>MEAVPRMPMIWLDLKEAGDFHFQPAVKKFVLKNYGENPEAYNEELKKLELLRQNAVRVPRDFEGCSVLRKYLGQLHYLQSRVPMGSGQEAAVPVTWTEIFSGKSVAHEDIKYEQACILYNLGALHSMLGAMDKRVSEEGMKVSCTHFQCAAGAFAYLREHFPQAYSVDMSRQILTLNVNLMLGQAQECLLEKSMLDNRKSFLVARISAQVVDYYKEACRALENPDTASLLGRIQKDWKKLVQMKIYYFAAVAHLHMGKQAEEQQKFGERVAYFQSALDKLNEAIKLAKGQPDTVQDALRFTMDVIGGKYNSA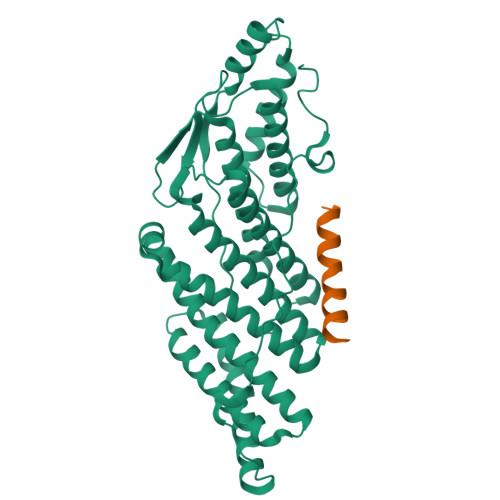KKDNDFIYHEAVPALDTLQPVKGAPLVKPLPVNPTDPAVTGPDIFAKLV[2x];>MDSYFKAAVSDLDKLLDDFEQN[2x]3-[3-(1~{H}-1,2,3,4-tetrazol-5-yl)phenyl]benzoic 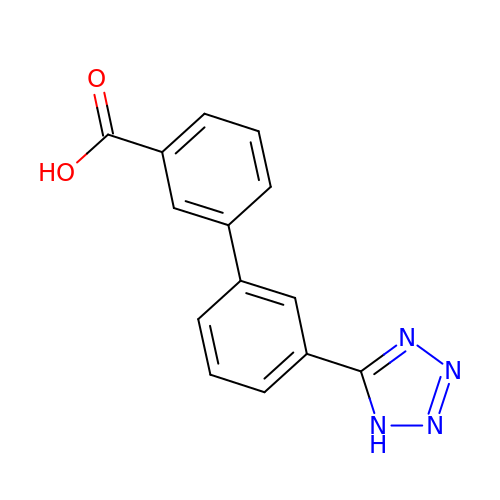acid | C14 H10 N4 O2 | KEZGIRGXOUGLEM-UHFFFAOYSA-N>ADSVIKSDFSSLKLDV[4x];>[4x]LERRTFGSYKIEELTIRNDQPTRNTNLSLSQSTENRLSTKKIPLLDDGIFELLNYLIDGTNFNKTCYCGFNYSHLPNLERDFNIASLYVRENFEICTDQLDLANYVRQPNISIKSPDFTVCLEYVLKTVVESESSTKDQKDDESQKPTSTDSTKNEQETKFVEMSLLPLLNRESEESLTEEILEGEGAVVNVLKLFIKGFL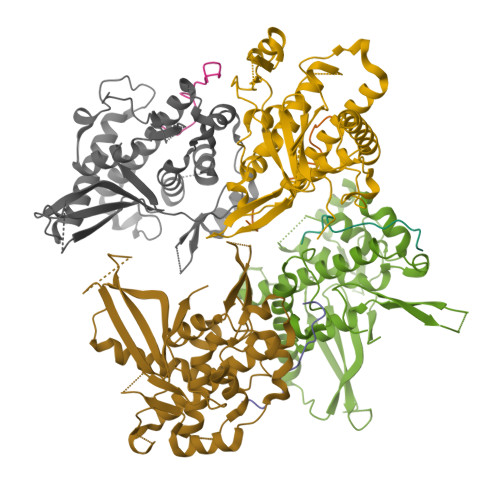MHLGENPNSYDRQLTVEKYRPLLVSIVGYEYLVGTTVPEKKINHIYYQLATFDNYPFDLLRFQLSSLISTPTSILERITKEGLFKIITSSTLRGAPRQTVLFRGINGSESFLNIKRYRRF~{N}4-(2,5-dimethoxyphenyl)-~{N}2-(2-propan-2-ylsulfonylphenyl)-1,3,5-triazine-2,4-diamine | C20 H23 N5 O4 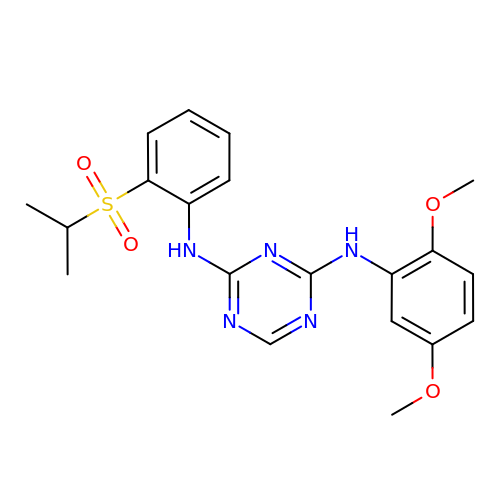S | PGEVTSPIPOQOQQ-UHFFFAOYSA-N>[6x]MSAAPVLSITNASVVYPDGISTVTALDSANVEIFPGELVAIVGESGSGKSTLLSIAGFLQEPTSGTVTLHGAEGLDATSTRREHIGFVFQQPNLLGSLTAREQLLITDHLRGIKPRKDRADELLARVGLKGLGGRRVAQLSGGQRQRVNIARALMGNPQLLLADEPTSALDARLSKEIVELLRDVTKEFALATLMVTHDRSQLAYADRFVEMADGKALQTAKLWSHPQFEK;>MFLGIRDIRAAAGRFALIASVVGLITLLIVMLTGLTQGLGKQNTSAIEALAPHSVVFTTAGGSSPEFTSSEISEQQAERWKDSTPLGVSQTRIESDQNANTTAVMGLPEGTPLPDSVGGFIEQGALLPAELADFLHVRAGDHITLGGATVTVAGTVKTENYSHTPVVWVDTATWQLVSHTKAVGTVLLLNQEPTIQPQDNEVVTDLKGAFQAMPAYKSE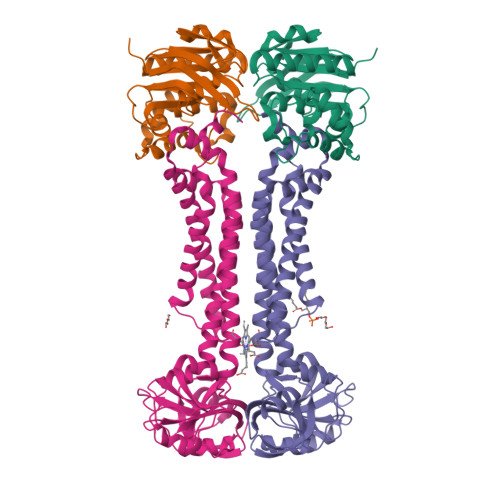RSSLLSMQAFLYIISALVTVAFLTVWTLQRTRDIAVLAALGASKRYLLIDALGQAAIILAAGVALGAGIGALLGWLIAGSVPFSLGWVSVLGPALGIWLLGLIGATIAVRNVTKVDPQIALGATA[6x]>[4x]MEQTYFISGANRGIGFSVVQRLAAKSGVKVIATARD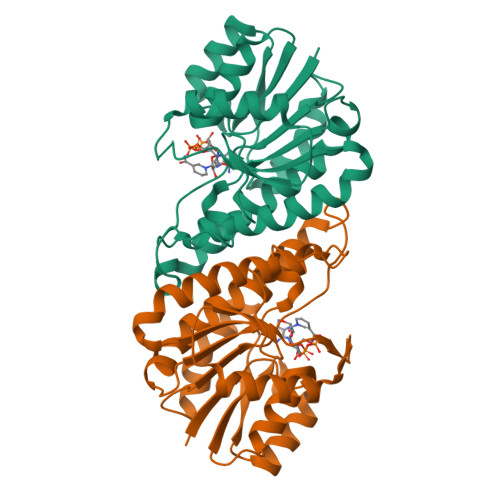PASATALNELAKENPQVKVVQLDISDEESIKKIAKNVSQYTDSIDVFVSNAAIAKSFGPLLNTPREQWIEHFFTNVLGPIRLFQELYPLIKKGTQKKVFFISSNAGSLNLDFGLDFSAFGQSKAALNYSTKELARQLKPENFIVAAVHPGKVTTDMGKGGERAFTAVDEVSAKKFFTPETKITPEESAAALCKLFESLNTTGKYLSYDGTELPW> MDGSGEQPRGGGPTSSEQIMKTGALLLQGFIQDRAGRMGGEAPE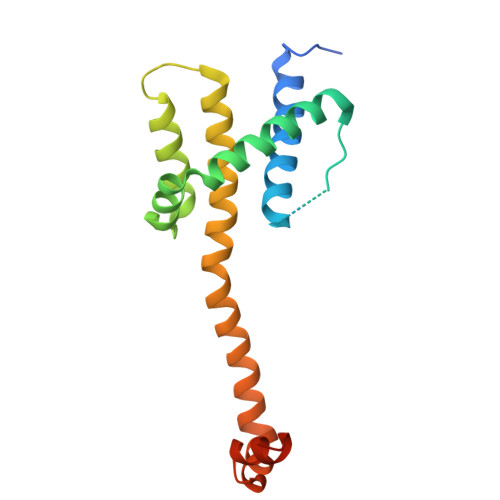LALDPVPQDASTKKLSESLKRIGDELDSNMELQRMIAAVDTDSPREVFFRVAADMFSDGNFNWGRVVALFYFASKLVLKALSTKVPELIRTIMGWTLDFLRERLLGWIQDQGGWDGLLSYFGTPTWQGSS> MAQTVPYGIPLIKADKVQAQGFKGANVKVAVLDTGIQASHPDLNVVGGASFVAGEAYNTDGNGHGTHVAGTVAALDNTTGVLGVAPSVSLYAVKVLNSSGSGSYSGIVSGIEWATTNGMDVINMSLGGASGSTAMKQAVDNAYARGVVVVAAAGNSGSSGNTNTIGYPAKYDSVIAVGAVDSNSNRASFSSVGAELEVMAPGAGVYSTYPTNTYATLNGTSMASPHVAGAAALILSKHPNLSASQVR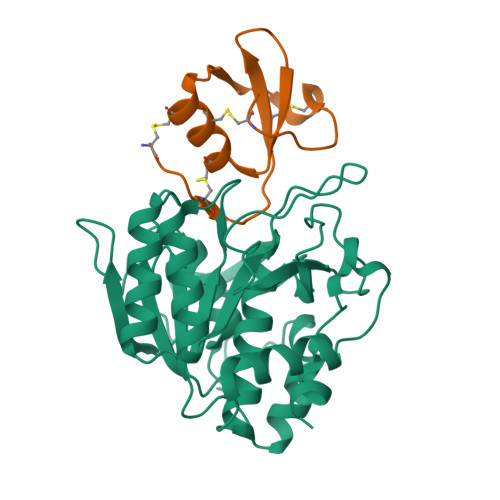NRLSSTATYLGSSFYYGKGLINVEAAAQ;> SEDDGSASPESQEMSYTELPCPSICPLIYAPVCVEDSNQDFYLFVNECEVRKCGCEAGFVYTFVPREMCKATTSLCPMQTKSS> MSIVTKSIVNADAEARYLSPGELDRIKAFVTGGAARLRIAETLTGSRETIVKQAGDRLFQKRPDIVSPGGNAYGEEMTATCLRDMDYYLRLVTYGVVSGDVTPIEEIGLVGVREMYRSLGTPIEA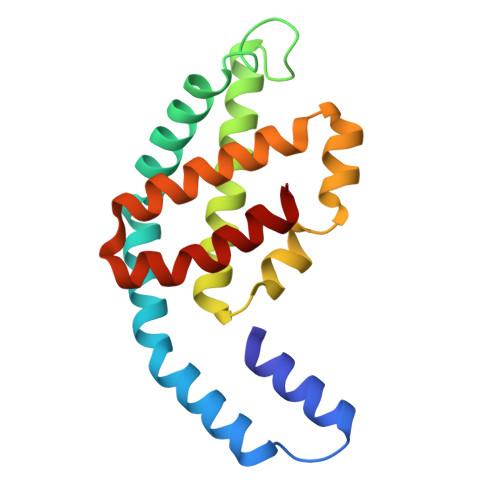VAQSVREMKEVASGLMSSDDAAEASAYFDFVIGKMS(1~{R},9~{S})-5-(3-oxidanylpropyl)-7,11-diazatricyclo[7.3.1.0^{2,7}]trideca-2,4-dien-6-one 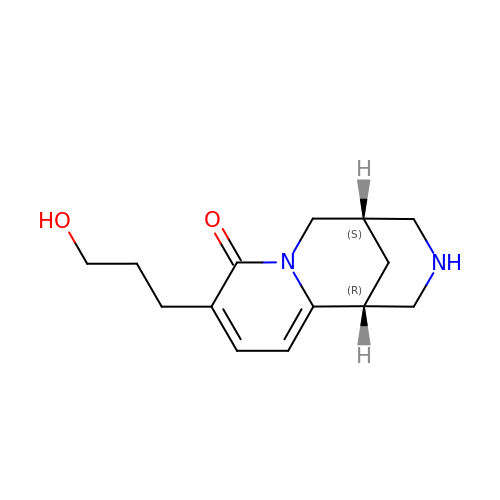| C14 H20 N2 O2 | JXEXVCIRYVIYEW-CMPLNLGQSA-N>KPRQKRTATKAYNVTQAFGRRGPEQTQGNFGDQELIRQGTDYKHWPQIAQFAPSASAFFGMSRIGMEVTPSGTWL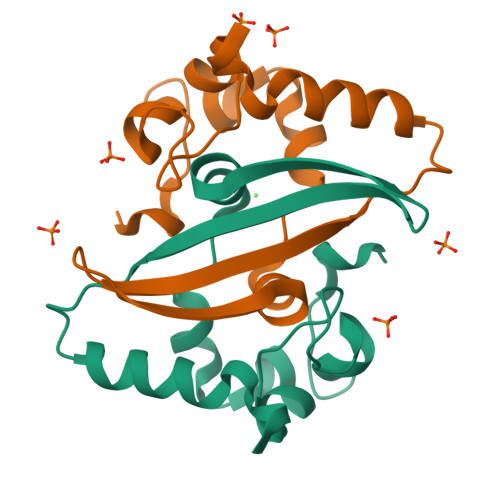TYTGAIKLDDKDPNFKDQVILLNKHIDAYKT[2x]> SIERLGYLGFAVKDVPAWDHFLTKSVGLMAAGSAGDAALYRADQRAWRIAVQPGELDDLAYAGLEVDDAAALERMADKLRQAGVAFTRGDEALMQQRKVMGLLCLQ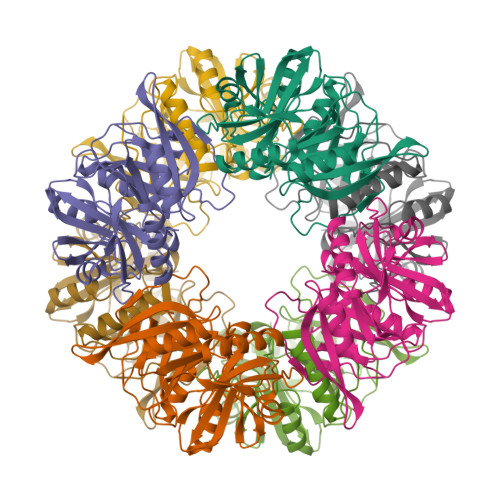DPFGLPLEIYYGPAEIFHEPFLPSAPVSGFVTGDQGIGAFVRCVPDTAKAMAFYTEVLGFVLSDIIDIQMGPETSVPAHFLHCNGRHHTIALAAFPIPKRIHHFMLQANTIDDVGYAFDRLDAAGRITSLLGRHTNDQTLSFYADTPSPMIEVEFGWGPRTVDSSWTVARHSRTAMWGHKSVRGQR>MS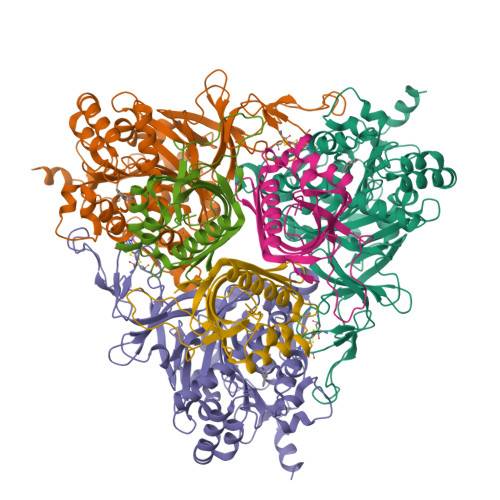SDATLVDTVNASQSRQVFWDEDVYALEIERIFSRAWLMLGHESLVPKPGDFITTYMAEDKVILSHQSDGTFRAFINSCSHRGNQICHADSGNAKAFVCNYHGWVFGQDGSLVDVPLESRCYHNSLDKQKLAAKSVRVETYKGFIFGCHDPEAPSLEDYLGEFRYYLDTIWEGAGGGMELLGPPMKSLLQCNWKVPAENFIGDGYHVGWTHAAALSQIGGELAGLAGNRADIPFDDLGLQFTTRHGHGFGVIDNAAAGLHIKREGWTKFLEDTRGEVRRKFGPERERLYLGHWNCSIFPNCSFLYGTNTFKIWHPRGPHEIEVWTYTIVPRDADPATKSMIQREAIRTFGTAGTLESDDGENMSSATYINRGVITRNGRMNSTMGVGYEGPHPVYPGIVGISFIGETSYRGFYRFWKEMIDAPDWASVKANDDTWDSVFPNRNFWNEKLNAAE[3x];>[3x]MSSEQIPVTPDVHYDIEAHYRAEVRMFQTGQYREWLQGMVAEDIHYWMPIYEQRLTRDRRPDPTPDDAAIYNDDFGELKQRVERLYSGQVWMEDPPSKIRYFVSNVEAFEAGNGELDVLSNILVYRNRRQTEVTVHTLGREDKLRRDGNGFKVFRRKLILDARVTQDKNLYFFC> MARQNLKSTDRAVQQMLDKAKREGIQTVWDRYEAMKPQCGFGETGLCCRHCLQGPCRINPFGDEPKVGICGATAEVIVARGLDRSIAAGAAGHSGDAKHLAHTLKKAVQGKAASYMIKDRTKLHSIAKRLGIPTEGQKDEDIALEVAKAALADFHEKDTPVLWVTTVLPPSRVKVLSAHGLIPAGIDHEIAEIMHRTSMGCDADAQNLLLGGLRCSLADLAGCYMGTDLADILFGTPAPVVTESNLGVLKADAVNVAVHGHNPVLSDIIVSVSKEMENEARAAGATGINVVGICCTGNEVLMRHGIPACTHSVSQEMAMITGALDAMILDY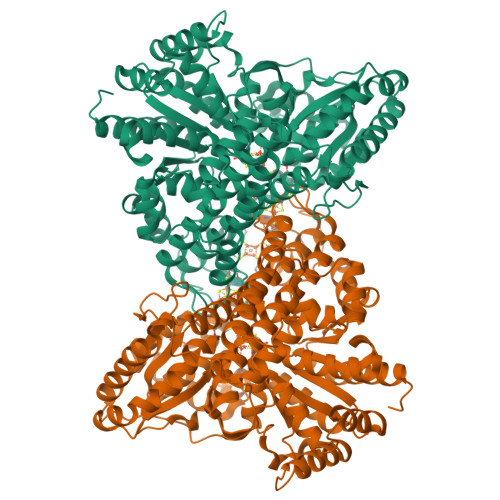QCIQPSVATIAECTGTTVITTMEMSKITGATHVNFAEEAAVENAKQILRLAIDTFKRRKGKPVEIPNIKTKVVAGFSTEAIINALSKLNANDPLKPLIDNVVNGNIRGVCLFAGCNNVKVPQDQNFTTIARKLLKQNVLVVATGCGAGALMRHGFMDPANVDELCGDGLKAVLTAIGEANGLGGPLPPVLHMGSCVDNSRAVALVAALANRLGVDLDRLPVVASAAEAMHEKAVAIGTWAVTIGLPTHIGVLPPITGSLPVTQILTSSVKDITGGYFIVELDPETAADKLLAAINERRAGLGLPW>[2x]AHCTEYMNAPKKLPADVAEELATTAQKLVQAGKGILAADESTQTIKKRFDNIKLENTIENRASYRDLLFGTKGLGKFISGAILFEETLFQKNEAGVPMVNLLHNENIIPGIKVDKGLVNIPCTDEEKSTQGLDGLAERCKEYYKAGARFAKWRTVLVIDTAKGKPTDLSIHETAWGLARYASICQQNRLV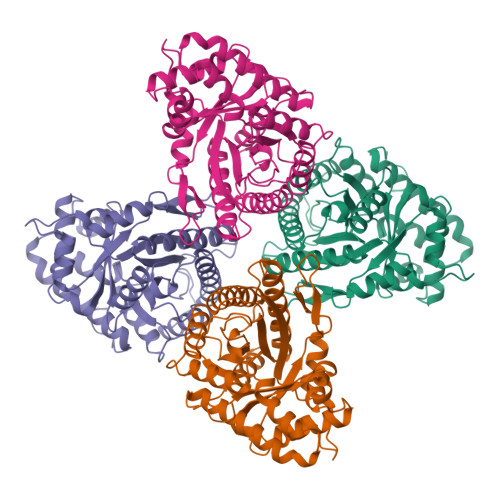PIVEPEILADGPHSIEVCAVVTQKVLSCVFKALQENGVLLEGALLKPNMVTAGYECTAKTTTQDVGFLTVRTLRRTVPPALPGVVFLSGGQSEEEASVNLNSINALGPHPWALTFSYGRALQASVLNTWQGKKENVAKAREVLLQRAEANSLATYGKYKGGAGGENAGASLYEKKYVY Acid ceramidase (aCDase; ASAH1) is the best studied member of the family and is prominent for its involvement in Farber disease (FD), a genetic disorder in humans. aCDase is ubiquitously expressed and found in the lysosome where it normally regulates sphingolipid metabolism through intralysosomal membrane turnover. Similar to other Ntn-hydrolases, aCDase is synthesized as an inactive proenzyme that requires proteolysis for activation. The α-subunit consists of a globular helical domain formed by five α-helices preceded by a 36-residue linker region, whereas the β-subunit contains two central anti-parallel β-sheets flanked on either side by a total of six α-helices.

Two structures are of the full-length proenzyme before autocleavage, from naked mole rat (nmr, 83% identity to human) and common minke whale (cmw, 85% identity). The autocleavage reaction was prevented in these structures by mutating the catalytic cysteine residue to alanine (C143A). Although the overall structures of the proenzymes from nmr-aCDase and cmw-aCDase are similar (root-mean-square deviation (r.m.s.d.) = 0.73 Å), there are differences. In the α-subunit, the orientations and lengths of helices, particularly helices-α2 and -α3, are slightly different. The β-subunits are essentially identical, but there is a significant deviation in the ~ 14-residue loop connecting strand-β4 to helix-α6 (L4-6). In nmr-aCDase, L4-6 forms an extended structure that protrudes ‘outward,’ whereas in cmw-aCDase it flips toward the center of the protein and sits atop the junction between the subunits. The significance of this loop variation is unclear, because in cmw-aCDase it is involved in a crystal contact. In the proenzyme structure, the peptide bond between Cys 143 (Ala 143 in the inactivated structures) and residue 142 (methionine in nmr-aCDase and isoleucine in cmw-aCDase) is intact as shown by continuous electron density. Since both inactive structures are of the C143A mutant, the position of the thiol was not experimentally determined, but we could model it based on energetically accessible cysteine rotamers and their corresponding steric clashes with the protein. In both inactive structures, only one rotamer satisfies these criteria (Rot1).

>DRHHHHHHKLQHVPPWTEDCRKSTYPPSGPTYRGPVPWYTINLDLPPYKRWHELMVDKAPALKVIVNYLKNMINAFEPSGKIVQLVDQKLPGLLGSFPGPFEEEMKGIAAVTEIPLGEIILFNIFYEFFTIATSIITEDKEGHLLHARNMDFGVFLGWNVNNNTWVVTEELKPLTVNLDFQRNSKTVFKAAGFAGYVGMLTGFKPGLFSLTLNERFSTNGGFMGVIEWILGKKDAKWIGFIIRSVLENSTSYEEAKTILTKSKILAPAYFILGGSKSGEGCVITRDRVQSLDIYELDPKQGIWYVVQTNYDRWKNPFFLDNRRTPAKMCLNRTTQENISFATMYDVLSTKPVLNKLTVYTALIDVTKGQFETYLRDCPDPCIGW[2x]> MSKLLMIGTGPVAIQLANICYLKSDYEIDMVGRASTSEKSKRLYQAYKKEKQFEVKIQNEAHQHLEGKFEINRLYKDVKNVKGEYETVVMACTADAYYDTLQQLSLETLQSVKHVILISPTFGSQMIVEQFMSKFSQDIEVISFSTYLGDTRIVDKEAPNHVLTTGVKKKLYMGSTHSNSTMCQRISALAEQLKIQLEVVESPLHAETRNSSLYVHPPLFMNDFSLKAIFEGTDVPVYVYKLFPEGPITMTLIREMRLMWKEMMAILQAFRVPSVNLLQFMVKENYPVRPETLDEGDIEHFEILPDILQEYLLYVRYTAILIDPFSQPDENGHYFDFSAVPFKQVYKNEQDVVQIPRMPSEDYYRTAMIQHIGKMLGIKTPMIDQFLTRYEASCQAYKDMHQDQQLSSQFNTN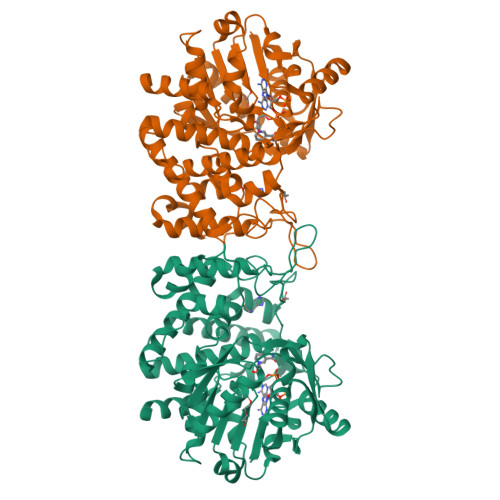LFEGDKALVTKFLEINRTLSLEHHHHHH> APTATLANGDTITGLNAIINEAFLGIPFAEPPVGNLRFKDPVPYSGSLDGQKFTSYGPSCMQQNPEGTYEENLPKAALDLVMQSKVFEAVSPSSEDCLTINVVRPPGTKAGANLPVMLWIFGGGFEVGGTSTFPPAQMITKSIAMGKPIIHVSVNYRVSSWGFLAGDEIKAEGSANAGLKDQRLGMQWVADNIAAFGGDPTKVTIFGESAGSMSVMC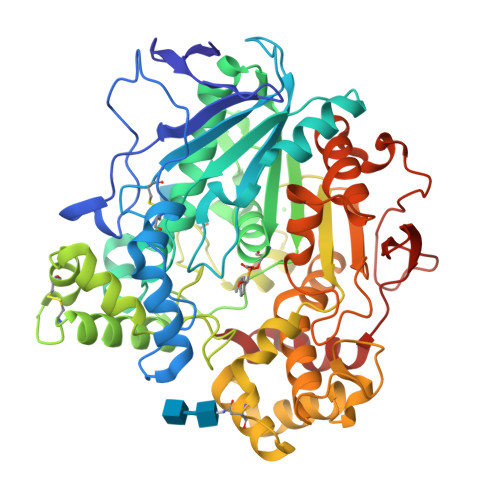HILWNDGDNTYKGKPLFRAGIMQSGAMVPSDAVDGIYGNEIFDLLASNAGCGSASDKLACLRGVSSDTLEDATNNTPGFLAYSSLRLSYLPRPDGVNITDDMYALVREGKYANIPVIIGDQNDEGTFFGTSSLNVTTDAQAREYFKQSFVHASDAEIDTLMTAYPGDITQGSPFDTGILNALTPQFKRISAVLGDLGFTLARRYFLNHYTGGTKYSFLSKQLSGLPVLGTFHSNDIVFQDYLLGSGSLIYNNAFIAFATDLDPNTAGLLVKWPEYTSSSQSGNNLMMINALGLYTGKDNFRTAGYDALFSNPPSFFV> GDTETAIDNAIARVADTVASGPSNSTSIPALTAVETGHTSQVEPSDTMQTRHVKNYHSRSESTVENFLSRSACVYIEEYYTKDQDNVNRYMSWTINARRMVQLRRKFELFTYMRFDMEITFVITSRQLPGTSIAQDMPPLTHQIMYIPPGGPVPNSVTDFAWQTSTNPSIFWTEGNAPPRMSIPFISIGNAYSNFYDGWSHFSQNGVYGYNALNNMGKLYARHVNKDTPYQMSSTIRVYFKPKHIRVWVPRPPRLSPYIKSSNV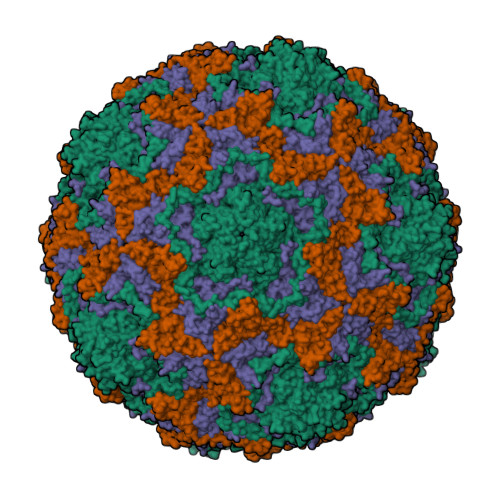NFNPTNLTDERSSITYVPDTIRPDVRTN;> PSAEECGYSDRVRSLTLGNSTITTQESANVVVGYGRWPEYLRDDEATAEDQPTQPDVATCRFYTLESVQWEKNSAGWWWKFPEALKDMGLFGQNMLYHYLGRAGYTIHVQCNASKFHQGCLLVVCVPEAEMGCSQTDKEVAAMNLTKGEAAHKFEPTKTNGEHTVQSIVCNAGMGVGVGNLTIYPHQWINLRTNNCATIVMPYVNSVPMDNMFRHYNFTLMVIPFAPLDYAAQASEYVPVTVTIAPMCAEYNGLRLAYQQ;> GLPVLNTPGSNQFMTSDDFQSPSAMPQFDVTPHMDIPGEVHNLMEIAEVDSVVPVNNIKANLQSMDAYHIEVNTGNYQGEKIFAFQMQPGLESVFKRTLMGEILNYYAHWSGSIKLTFTFCGSAMATGKLLLAYSPPGADVPATRKQAMLGTHMIWDIGLQSSCVLCIPWISQTHYRLVQQDEYTSAGNVTCWYQTGIVVPPGTPNKCVVLCFASACNDFSVRMLRDTPFIGQTALLQ;> MGAQVSTQKTGAHETGLNASGNSIIHYTNINYYKDAASNSANRQDFTQDPGKFTEPVKDIMIKTMPALNS>[4x]MSLNITGIQSDWKVEKIEFAKLTGERARSAGANGRIGVHGKSCTVDIARITIDGQTGYGSSIHMTPEWAEDVIGRRLLDLFDDRGRLREAYRLQLEYPVLDWLGQRQGKPVYDLVSGAHLETGASLVVPCYDTSLYFDDLHLADER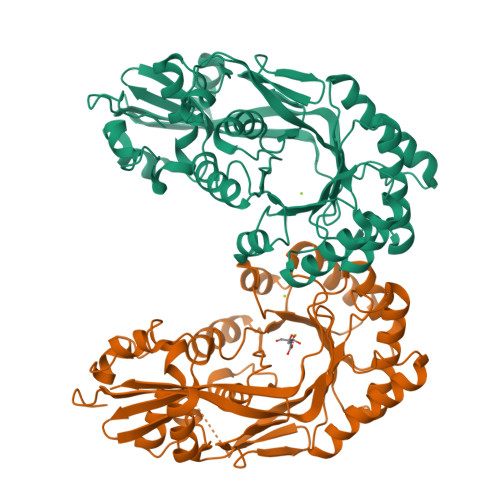AAVALMQEEAMQGYAKGQRHFKIKVGRGGRHMPLWEGTKRDIAIVRGISEVAGPAGKIMIDANNAYNLNLTKEVLAALSDVNLYWLEEAFHEDEALYEDLKEWLGQRGQNVLIADGEGLASPHLIEWATRGRVDVLQYDIIWPGFTHWMELGEKLDAHGLRSAPHCYGNAYGIYASGHLSAAVRNFEFVEYDDITIEGMDVSGYRIENGEIHVPATPGFGIVFDDELVTYLINRSGWSEGHHHHHH Recognition of viral RNAs by RLRs leads to the activation of mitochondrial antiviral signaling protein (MAVS; also known as IPS1, VISA and CARDIF). Activated MAVS triggers rapid production of type I interferons and proinflammatory cytokines. It consists of an N-terminal CARD domain, a proline-rich region (PRR) preceding a poorly structured middle segment, and a monotopic transmembrane (TM) domain at the very C-terminus. The N-terminal CARD domain of MAVS is necessary and sufficient for forming active MAVS aggregates.

At the inter-strand interface, the positive and negative charges are alternately distributed at two opposite ends of each CARD subunit, indicating that the inter-strand interaction is mainly electrostatic. The positively charged residues R37 in the 3rd helix (H3), R64 and R65 in the loop between the 4th and 5th helices (H4 and H5) from the CARD in a lower layer (purple in Figure 2B) are in close proximity to the negatively charged residues D23 in the loop between the 1st and 2nd helices (H1b and H2) and E26 in the 2nd helix (H2) of another CARD molecule (cyan in Figure 2B) in the upper layer. E26, R64 and R65 are highly conserved among MAVS molecules from different species, but D23 and R37 are less so. As an alternative verification of the key residues for MAVS CARD self-association, we searched for mutants that disrupt the CARD polymerization in E. coli. We performed random mutagenesis and screened for soluble CARD mutants by using a recently developed solubility screen. Our screen recognized multiple sites that are important for CARD oligomerization. Biochemical analysis confirmed that most mutants from the screen were expressed as soluble proteins, and eluted as homogenous monomers in gel-filtration chromatography. Almost all the mutations out of the solubility screen are conserved and at the protein surface. They can be mapped to the two interfaces identified in the cryoEM model.

> GPHMTVAEDKTFQYIRQHHSNFSRIHVLEILPYLSCLTTSDQDRLRATYERWGNQDTLLELFTSLRCRNGWVHSLIGALRACELSGLADEVARIYHS> GPLGSGGGTIAMLNEISSDTLEQLYSLAFNQYQSGKYEDAHKVFQALCVLDHYDSRFFLGL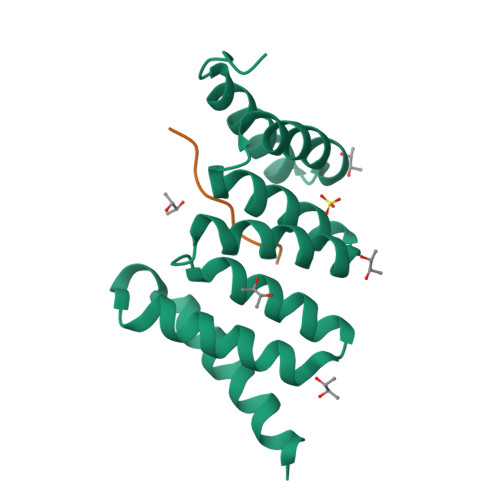GACRQAMGQYDLAIHSYSYGAVMDIKEPRFPFHAAECLLQKGELAEAESGLFLAQELIANKPEFKELSTRVSSMLEAIKLKKEMKHE;> XQVPELIKPSQ>[2x]SNATNIEAGKAQAAVSDKMDDQWKERVNPRKKLTPELGEAFARMYIPQFGSDFQFAIVEGTTDADLEAGPG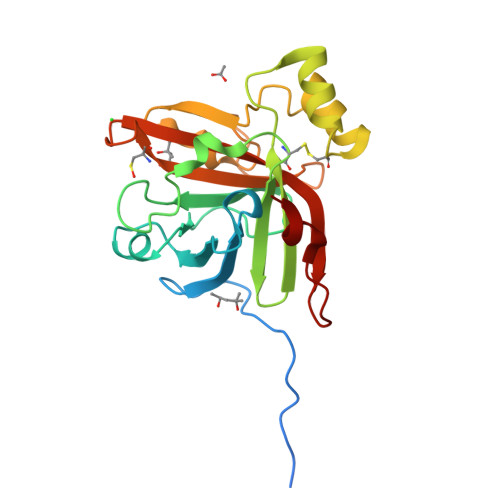HYNDTQLPGERGNFAVAGHRVGKGAPFNDLGNLNVCDAIVVETRTSWSVYRVMPVDSSGQQRYDEAMGCFTPEQAERITHGDYEHVNGRFITTPGDVSTISALPETDVIEADPGMEGIMTMTTCHPQFSNAERMIVHAMLTEHFPKNGDNKPAALEEG> MNTLANIQELARALRNMIRTGIIVETDLNAGRCRVQTGGMCTDWLQWLTHRAGRSRTWWAPSVGEQVLILAVGGELDTAFVLPGIYSGDNPSPSVSADALHIRFPDGAVIEYEPETSALTVSGIKTASVTASGSVTATVPVVMVKASTRVT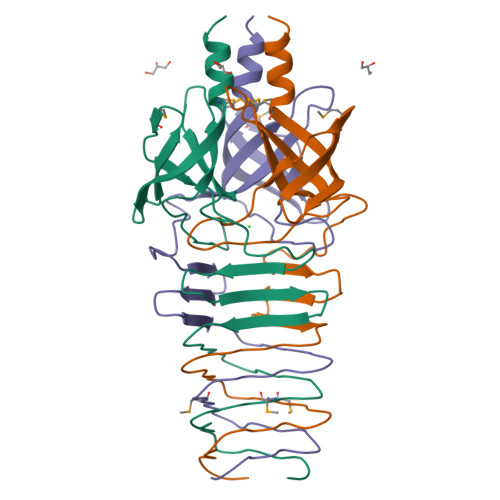LDTPEVVCTNRLITGTLEVQKGGTMRGNIEHTGGELSSNGKVLHTHKHPGDSGGTTGSPL>[2x]ADTIVAVELDSYPNTDIGDPN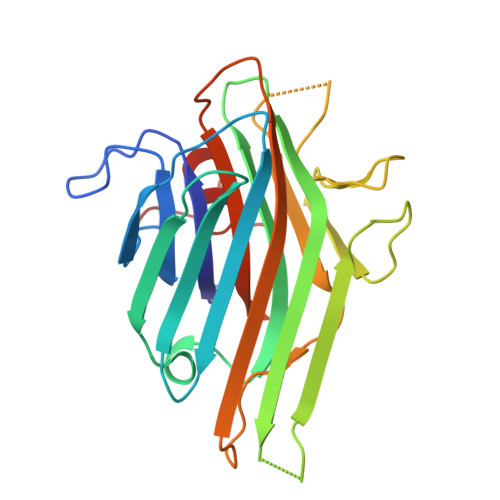YPHIGIDIKSIRSKSTARWNMQTGKVGTVHISYNSVAKRLSAVVSYSGSSSTTVSYDVDLNNVLPEWVKVGLSATTGLYKETNTILSWSFTSKLKTNSAADANSLHFSFNKFSQNPKDLILQGDAFTDSDGNLQLTKVSSSGDPQGNSVGRALFYAPVHIWEKSAVVASFDATFTFLIKSPDREPADGITFFIANTDTSIPSGSGGRLLGLFPDAN>[4x]MAEIKITPEELERIAGNFKNAAGEAQSQINRLEGDINSLE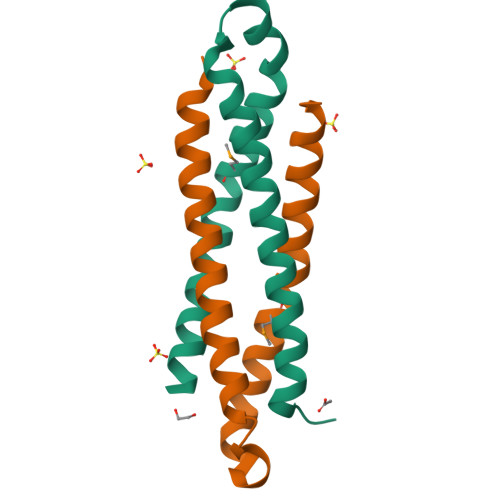GQWAGATQAKFRGEFIQSKQAMQQYIPILEGISTDLKRIADKFRNTDNAYAGHHHHHH1-(4-chlorophenyl)-N-methylmethanesulfonamide | C8 H10 Cl N O2 S | 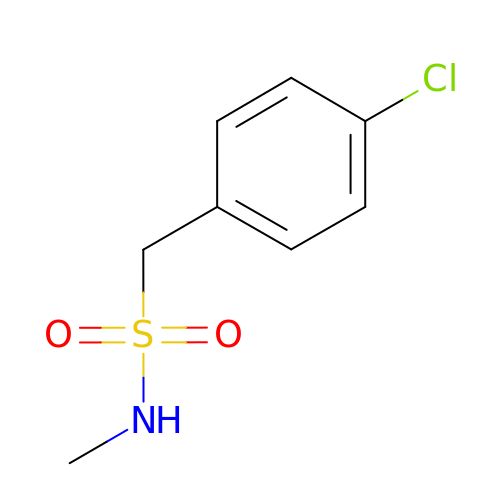YPYACBWYLBGTPU-UHFFFAOYSA-N> MSVTIDHTTENAAPAQAPVSDRAWALFRALDGKGLVPDGYVEGWKKTFEEDFSPRRGAELVARAWTDPEFRQLLLTDGTAAVAQYGYLGPQGEYIVAVEDTPTLKNVIVCSLCSCTAWPILGLPPTWYKSFEYRARVVREPRKVLSEMGTEIASDIEIRVYDTTAETRYMVLPQRPAGTEGWSQEQLQEIVTKDCLIGVAIPQVPTV;> MDGVHDLAGVQGFGKVPHTVNADIGPTFHAEWEHLPYSLMFAGVAELGAFSVDEVRYVVERMEPRHYMMTPYYERYVIGVATLMVEKGILTQDELESLAGGPFPLSRPSESEGRPAPVETTTFEVGQRVRVRDEYVPGHIRMPAYCRGRVGTISHRTTEKWPFPDAIGHGRNDAGEEPTYHVKFAAEELFGSDT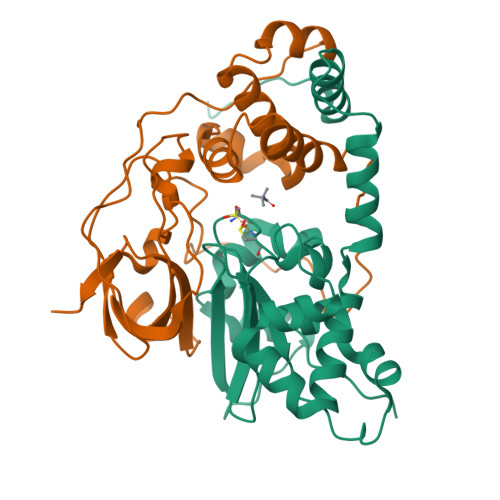DGGSVVVDLFEGYLEPAA> GSNNVLPTWSLDSNGEMRSRLSLSEVLDSGDLMKFAVDKTGCQFLEKAVKGSLTSYQ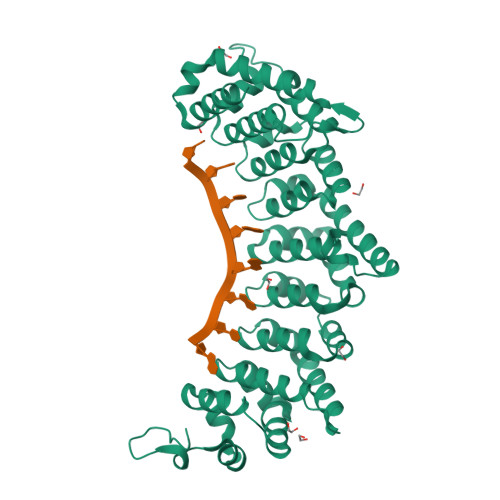KFQLFEQVIGRKDDFLKLSTNIFGNYLVQSVIGISLATNDDGYTKRQEKLKNFISSQMTDMCLDKFACRVIQSSLQNMDLSLACKLVQALPRDARLIAICVDQNANHVIQKVVAVIPLKNWEFIVDFVATPEHLRQICSDKYGAYVVSTIIEKLTADSMNVDLTSAAQNLRERALQRLMTSVTNRCQELATNEYANYIIQHIVSNDDLAVYRECIIEKCLMRNLLSLSQEKFASHVVEKAFLHAPLELLAEMMDEIFDGYIPHPDTGKDALDIMMFHQFGNYVVQCMLTICCDAVSGRRQTKEGGYDHAISFQDWLKKLHSRVTKERHRLSRFSSGKKMIETLANLRSTHPIYELQ> QDTSPDTLVVTANRFEQPRSTVLAPTTVVTRQDIDRWQSTSVNDVLRRLPGVDITQNGGSGQLSSIFIRGTNASHVLVLIDGVRLNLAGVSGSADLSQFPIALVQRVEYIRGPRSAVYGSDAIGGVVNIITTRDEPGTEISAGWGSNSYQNYDVSTQQQLGDKTRVTLLGDYAHTHGYDVVAYGNTGTQAQTDNDGFLSKTLYGALEHNFTDAWSGFVRGYGYDNRTNYDAYYSPGSPLLDTRKLYSQSWDAGLRYNGELIKSQLITSYSHSKDYNYDPHYGRYDSSATLDEMKQYTVQWANNVIVGHGSIGAGVDWQKQTTTPGTGYVEDGYDQRNTGIYLTGLQQVGDFTFEGAAR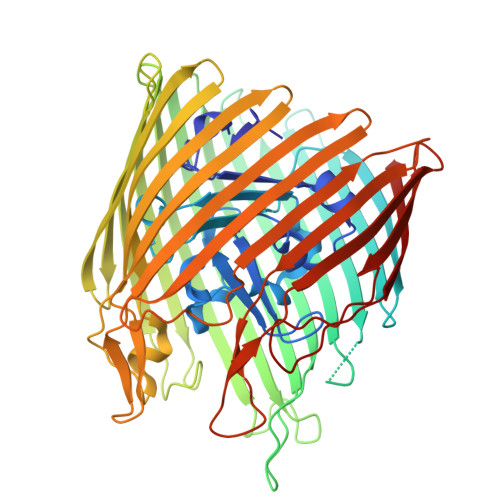SDDNSQFGRHGTWQTSAGWEFIEGYRFIASYGTSYKAPNLGQLYGFYGNPNLDPEKSKQWEGAFEGLTAGVNWRISGYRNDVSDLIDYDDHTLKYYNEGKARIKGVEATANFDTGPLTHTVSYDYVDARNAITDTPLLRRAKQQVKYQLDWQLYDFDWGITYQYLGTRYDKDYSSYPYQTVKMGGVSLWDLAVAYPVTSHLTVRGKIANLFDKDYETVYGYQTAGREYTLSGSYTF>SMWELTILHTNDVHSRLEQTSEDSSKCVDASRCMGGVARLFTKVQQIRRAEPNVLLLDAGDQYQGTIWFTVYKGAEVAHFMNALRYDAMALGNHEFDNGVEGLIEPLLKEAKFPILSANIKAKGPLASQISGLYLPYKVLPVGDEVVGIVGYTSKETPFLSNPGTNLVFEDEITALQPEVDKLKTLNVNKIIALGHSGFEMDKLIAQKVRGVDVVVGGHSNTFLYTGNPPSKEVPAGKYPFIVTSDDGRKVPVVQAYAFGKYLGYLKIEFDERGNVISSHGNPILLNSSIPEDPSIKADINKWRIKLDDYSTQEL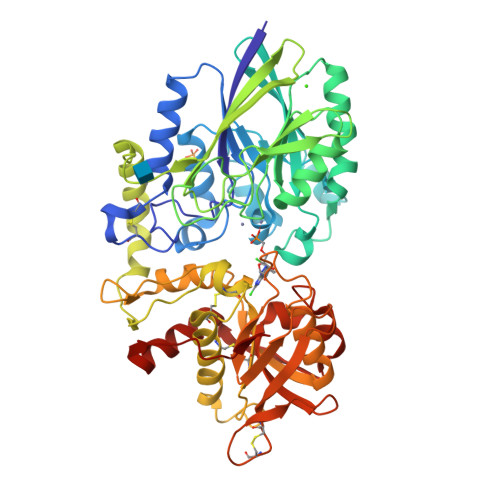GKTIVYLDGSSQSCRFRECNMGNLICDAMINNNLRHTDEMFWNHVSMCILNGGGIRSPIDERNDGTITWENLAAVLPFGGTFDLVQLKGSTLKKAFEHSVHRYGQSTGEFLQVGGIHVVYDLSRKPGDRVVKLDVLCTKCRVPSYDPLKMDEVYKVILPNFLANGGDGFQMIKDELLRHDSGDQDINVVSTYISKMKVIYPAVEGRIKFS[2x]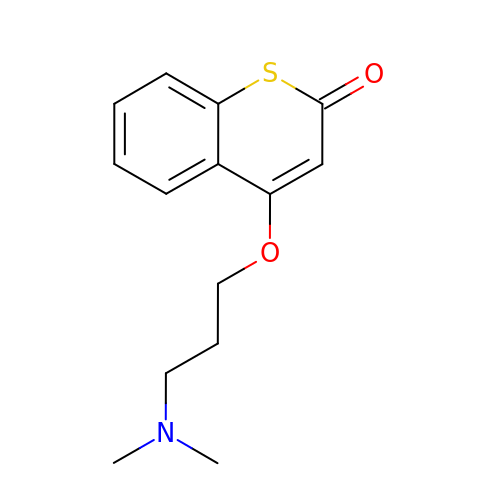THIOCOUMARIN | C14 H17 N O2 S | DIOZFKOOIBATNZ-UHFFFAOYSA-N>MATDLKASSLRALKLMHLATANDDDTDEKVIALCHQAKTPVGTTDAIFIYPRFIPIARKTLKEQGTPEIRIWTSTNFPHGNDDIDIALAETRAAIAYGADGVAVVFPYRALMAGNEQVGFDLVKACK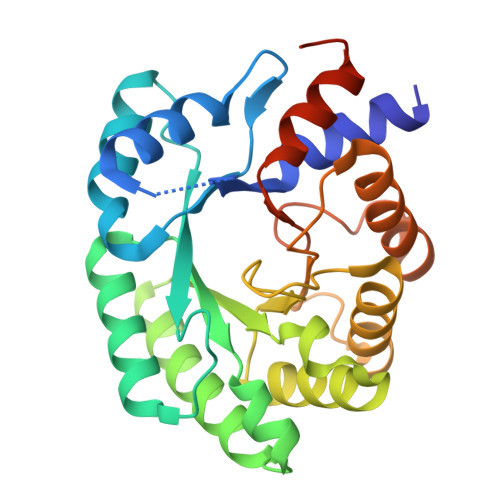EACAAANVLLSVIIETGELKDEALIRKASEISIKAGADHIVTSTGKVAVGATPESARIMMEVIRDMGVEKTVGFIPAGGVRTAEEAQKYLAIADELFGADWADARHYAFGASSLLASLLKALGHGDGKSASSYGSLE[2x]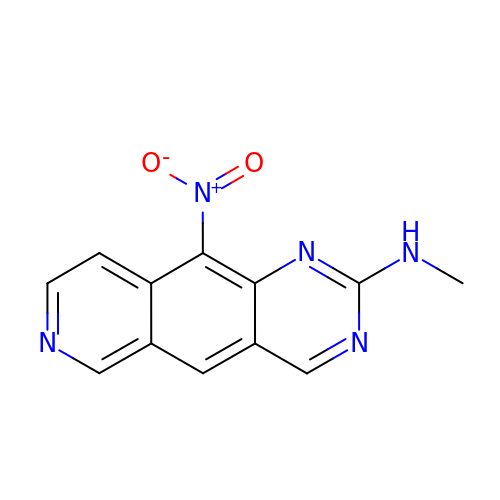~{N}-methyl-10-nitro-pyrido[3,4-g]quinazolin-2-amine | C12 H9 N5 O2 | WJQCMHKMNXKJQR-UHFFFAOYSA-N>SAGAHAGWETPEGCEQVLTGKRLMQCLPNPEDVKMALEVYKLSLEIEQLELQRDSARQSTLDKEL[7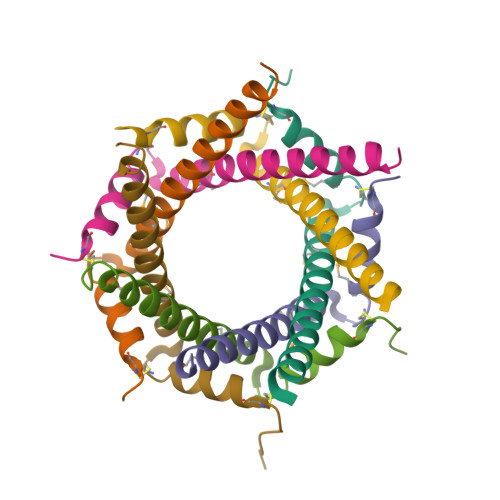x]> SSLDDKPQFPGASAEFIDKLEFIQPNVISGIPIYRVMDRQGQIINPSEDPHLPKEKVLKLYKSMTLLNTMDRILYESQRQGRISFYMTNYGEEGTHVGSAAALDNTDLVFGQYREAGVLMYRDYPLELFMAQCYGNISDLGKGRQMPVHYGCKERHFVTISSPLATQIPQAVGAAYAAKRANANRVVICYFGEGAASEGDAHAGFNFAATLECPIIFFCRNNGYAISTPTSEQYRGDGIA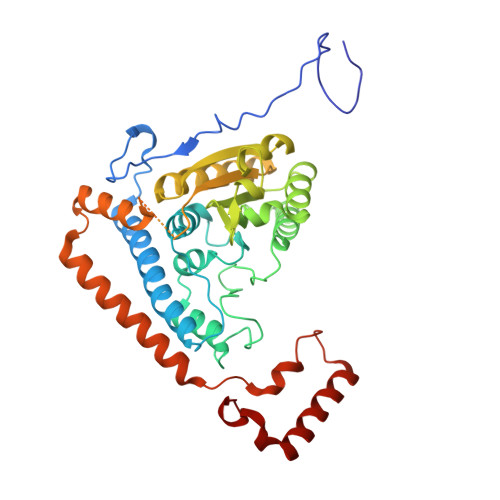ARGPGYGIMSIRVDGNDVFAVYNATKEARRRAVAENQPFLIEAMTYRIGHASTSDDSSAFRSVDEVNYWDKQDHPISRLRHYLLSQGWWDEEQEKAWRKQSRRKVMEAFEQAERKPKPNPNLLFSDVYQEMPAQLRKQQESLARHLQTYGEHYPLDHFDK>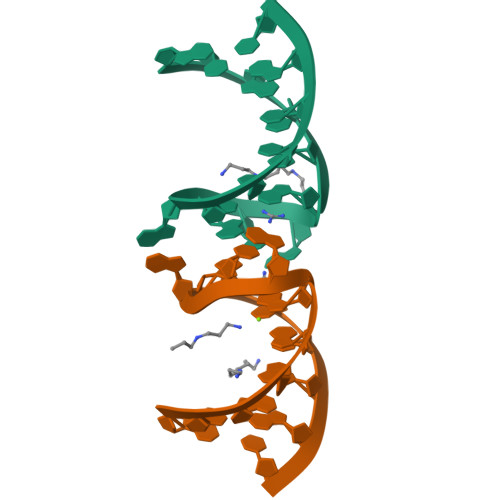GCGGGGACGACCCUGC[4x]>[5x]VRTCLPCGPGGKGRCFGPSICCGDELGCFVGTAEALRCQEENYLPSPCQSGVKPCG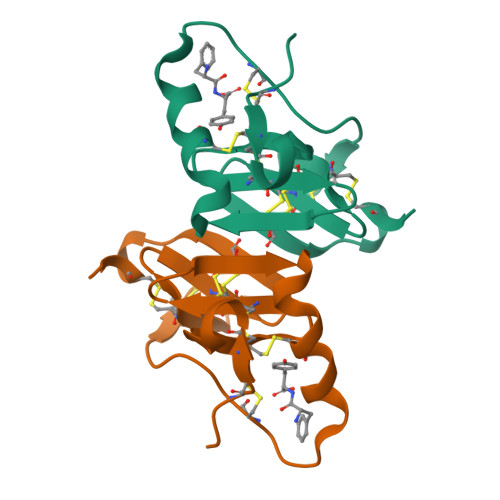SGGRCAAAGICCSPDGCHEDPACDP>[2x]SDTVIIAGGGPVGLMLACELGLAGVDTVVLERHDAPREPSRGGAINATVVELFTQRGIMESLRDDGFEFRMAHFAHI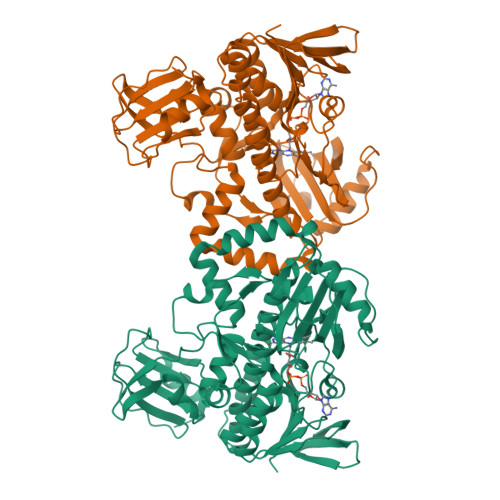PLAPERVPGDRAFSFAVPHAQVERRLEERARSLGVRVRRSTEITSVRQTPDGVQVTTGDGEVVEGAYLVGCDGSASLVREQAGIPFPGVDPDFHGLWGDIKVEPGAPVLERIGARQYELGLCMVAPIGPDTVRVITGEFDVPSPPADQEVGFDELRAAVARIAGVELDGVPGWLSRWTATSRQAERYREGRILLAGDAAHTLFPLGGQALGTGIEDAVNLGWKLAATVQGWAPPSLLDSYHEERHAAGARACASTRAQTTIMRSLARVGELRALLTELAGLEEVNAYLVRMVGGIDGSRLPDVPLVTAEGETSVYRLLEAGRGVLLDLGAGLPAVRHPQVTYVRAEPTNRLDATAVLLRPDGVVAWRAPQDGLEAALETWFGPAA>GPMGMTLHATRGAALLSWVNSLHVADPVEA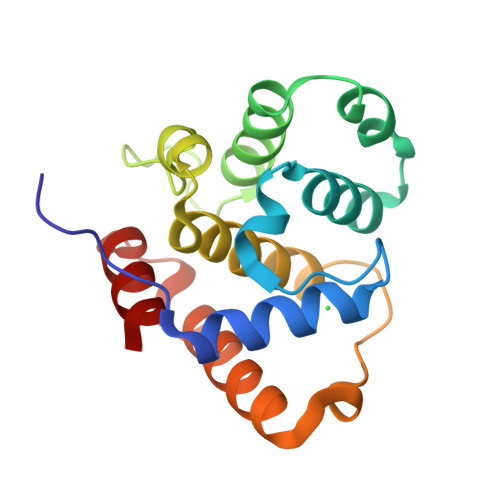VLQLQDCSIFIKIIDRIHGTEEGQQILKQPVSERLDFVCSFLQKNRKHPSSPECLVSAQKVLEGSELELAKMTMLLLYHSTMSSKSPRDWEQFEYKIQAELAVILKFVLDHEDGLNLNEDLENFLQK[4x]>MAPALVQRRKKVAMIGSGMIGGTMGYLCALRELADVVLYDVVKGMPEGKALDLSHVTSVVDTNVSVRAEYSYEAALTGADCVIVTAGLTKVPGKPDSEWSRNDLLPFNSKIIREIGQNIKKYCPKTFIIVVTNPLDCMVKVMCEASGVPTNMICGMACMLDSGRFRRYVADALSVSPRDVQATVIGTHGDCMVPLVRYITVNGYPIQKFIKDGVVTEKQLEEIAEHTKVSGGEIVRFLGQGSAYYAPAASAVAMATSFLNDEKRVIP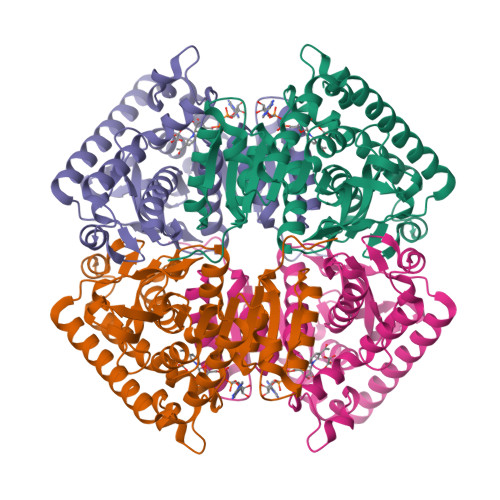CSVYCNGEYGLKDMFIGLPAVIGGAGIERVIELELNEEEKKQFQKSVDDVMALNKAVAALQAPG[4x]> MSSDPLQQVCDLIKGDLSLERVRDIKEQLLKEKSVVEYQLNKESDKYYGEVEESLKLLNLSKNSVTSIKQQINEVNKLGNDNRFAINRYDILFRATKLYETVNTTSSIYDRIYNFVALMEHIERLLVAELAEDALETGCPHLLEIHFLLTSARDFQEQVVVMAKEATEDAQRTVMKLFSRLSGIISKFDKLLDGLTYDIVEMARAEQISLAIRLFKIYDLEEREDLRIEAIRNIIKKKEIEIEKSSIKKLPNSKNTARLQDETPKVIEYPTNKGLYQEIMSGTISTRTAPRGYKHFLINGINNSISEMFGEMREKYVGDQKFDVLDNMDWIFNELIIVKEHIANCCPPHWNIFEVYFDQYYKELHSLITDLVESEPETIIILDILAFDKTFQDTLKQDFGFTKSEVKSVIGDKEKETLFKDYLNLIVVKMTEWIGNLEKAEFDVFLERSTPPHSDSDGLLFLDGTKTCFQMFT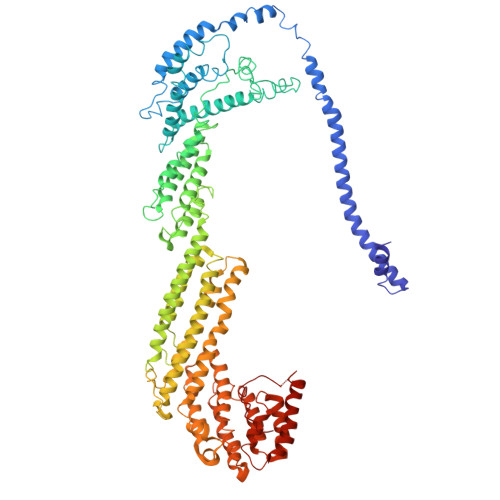QQVEVAAGTNQAKILVGVVERFSDLLTKRQKNWISKISEEIKKQINYNHKYDIDPESITPEDECPGGLVEYLIAVSNDQMKAADYAVAISSKYGKLVSKVYEKQITNHLEGTLDGFAEVAQCSSLGLITLMFDDLRKPYQEIFSKTWYMGSQAQQIADTLDEYLLDIKPQMNSVLFVNFIDNVIGETIIKFLTALSFEHSFKNKNNKFLEAMKRDFEIFYQLFVKVLDGNESKDTLITQNFTVMEFFMDLSCEPIDSILDIWQKYLEVYWDSRIDLLVGILKCRKDVSSSERKKIVQQATEMLHEYRRNMEANGVDREPTLMRRFVLEFEKQ>MRLKDLGERALLAR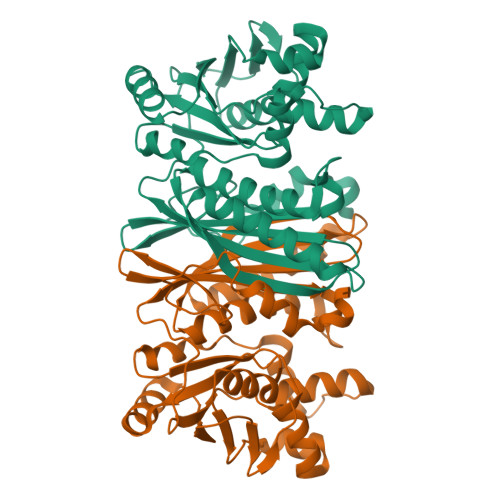LAPLGYPPEAPLPPGDDAGGVWAEGRAWLLKTDGFLYREVALKGMGPFEVGFRGVAATASDLLAKMGRPLGFTLGLFLPEDLEEGFVLELVRGAAEAAKRLGAFLLGGDTNRGVEVALTVSGYALAEAPLPRKALPGDLLYLAGDRWGRTGAAIRAHYEGRSLEGFPKIREAAFYPLPRLELLALSGLLRGSLDSSDGLAETLWQLADLGVGVEVEALPLYPDVLAFAGSEEAALELVLYGGEEFEAVLVVPQEGAAAVEARAKAKGLPLFRAGRVVAGEGVYLRGAPLPRKGYAHF[4x]N-{(1S)-1-[8-chloro-2-(3-fluorophenyl)quinolin-3-yl]ethyl}-9H-purin-6-amine | C22 H16 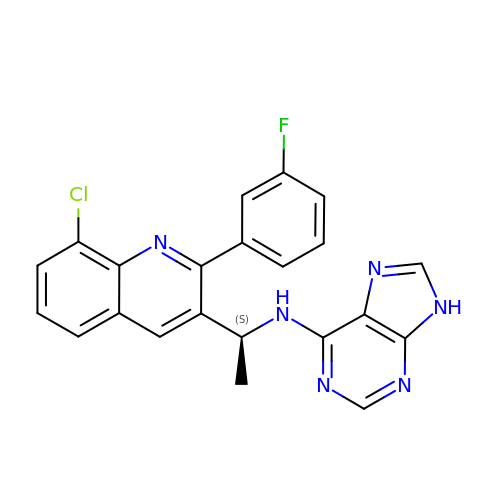Cl F N6 | OBNLXBLOBJTAKW-LBPRGKRZSA-N N-{[2-chloro-5-(2-{3-[4-(6-chloro-3-methyl-2-oxo-2,3-dihydro-1H-benzimidazol-1-yl)piperidin-1-yl]propyl}-3-oxo-2,3-dihydropyridazin-4-yl)phenyl]methyl}-4-fluorobenzamide | C34 H33 Cl2 F N6 O3 | 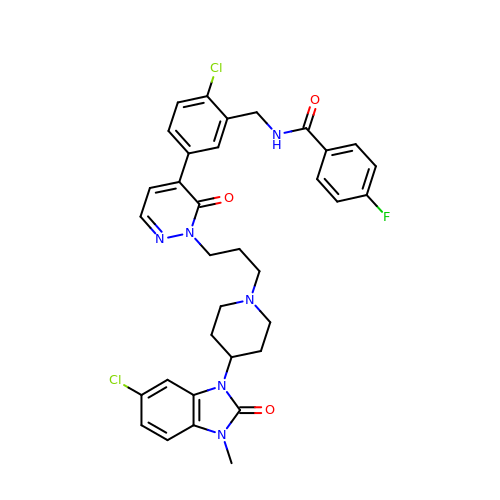LWFRBSJHBRLMJP-UHFFFAOYSA-N>GGGGGCCA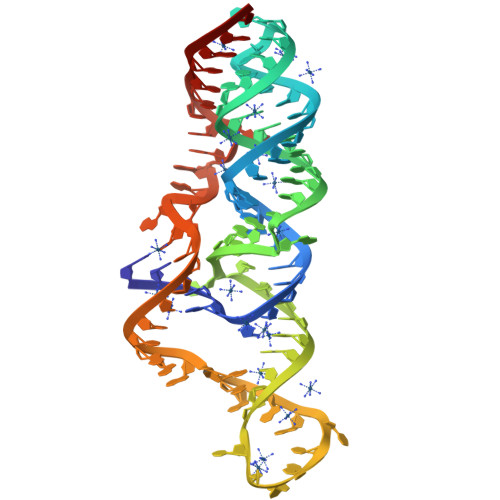GAUGUCAUGUCUCUCAAGCCUAGGAGACACUAGACACUCUGGACUAUCGGUUAGAGGAAACCCCCCCAAAAAUGUAUAGGCU[2x]> GSHM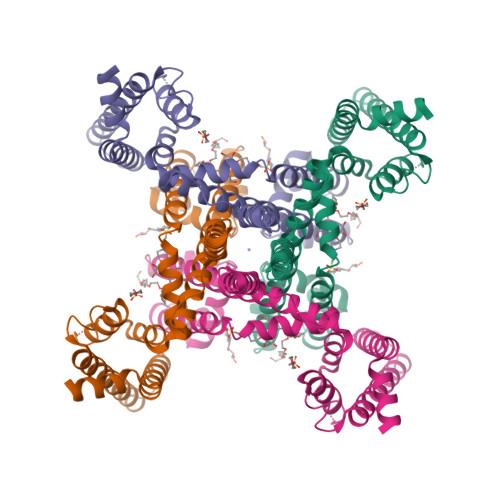SRKIRDLIESKRFQNVITAIIVLNGAVLGLLTDTTLSASSQNLLERVDQLCLTIFIVEISLKIYAYGVRGFFRSGWNLFDFVIVAIALMPAQGSLSVLRTFRIFRVMRLVSVIPTMRRVVQGMLLALPGVGSVAALLTVVFYIAAVMATNLYGATFPEWFGDLSKSLYTLFQVMTLESWSMGIVRPVMNVHPNAWVFFIPFIMLTTFTVLNLFIGIIVDAMAITKEQEEEAKTGHHQEPISQTLLHLGDRLDRIEKQLAQNNELLQRQQPQKK>[2x]MYEFKDYYQNTVQLSFDDQPFSDSPKHVWVICRFGGKWLLTEHEDRGYEFPGGKVEPMECAEEAALREVKEE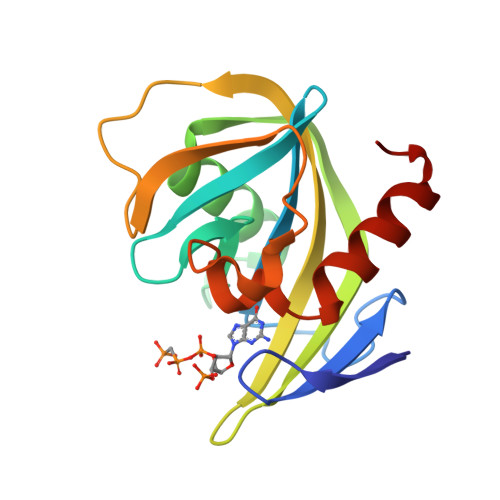TGARVKSLKYLGQYKVLGKEKVIVKNIYFADIEKLEKQADYFETKGPVLFHELPENLSRNKKFSFIMKDSVLPISLKKLKESGWIE> GTEAPDVDLADGNFYASREARAAYRWMRANQPVFRDRNGLAAASTYQAVIDAERQPELFSNAGGIRPDQPALPMMIDMDDPAHLLRRKLVNAGFTRKRVKDKEASIAALCDTLIDAVCERGECDFVRDLAAPLPMAVIGDMLGVRPEQRDMFLRWSDDLVTFLSSHVSQEDFQITMDAFAAYNDFTRATIAARRADPTDDLVSVLVSSEVDGERLSDDELVMETLLILIGGDETTRHTLSGGTEQLLRNRDQWDLLQRDPSLLPGAIEEMLRWTAPVKNMCRVLTADTEFHGTALC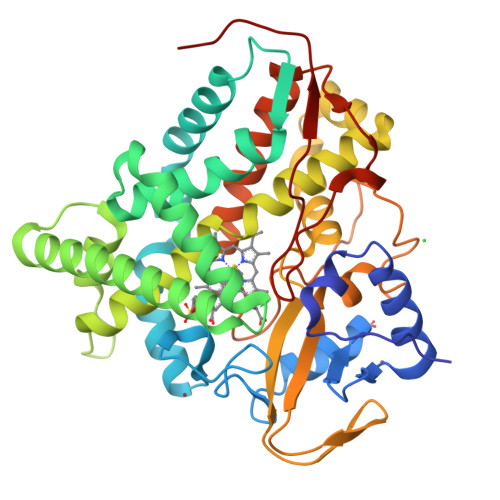AGEKMMLLFESANFDEAVFCEPEKFDVQRNPNSHLAFGFGTHFCLGNQLARLELSLMTERVLRRLPDLRLVADDSVLPLRPANFVSGLESMPVVFTPSPPLG MBTD1, Malignant Brain Tumor domain-containing protein 1, is one such PcG protein. MBTD1 is a four MBT repeat protein comprising 628 amino acids. It contains a FCS-type zinc finger at the N-terminus with putative regulatory function and four MBT repeats at the C-terminus. The MBT (Malignant Brain Tumor) repeat is a structural motif of ∼100 amino acids that is conserved from C. elegans to humans and exists as tandem repeats.

To investigate the crystal structure of the four MBT repeat fragment of MBTD1 and characterize its histone binding specificity, we cloned and purified a human MBTD1 fragment composed of all four MBT repeats (residues 130–566). MBTD1130–566 crystallized in the orthorhombic space group P212121 (a = 70.31 Å, b = 100.90 Å, c = 135.30 Å) with two molecules in the asymmetric unit. In the MBTD1 structure, each molecule contains four MBT repeats that exhibit irregular rhomboid architecture. A narrow channel runs through the middle of the structure and is filled with water molecules. Consistent with previously reported MBT repeat structures, each MBT repeat contains an extended “arm” which packs against a globular β subunit core of the preceding repeat. The residues involved in intermolecular hydrogen bond interactions between the two molecules in the asymmetric unit are conserved throughout the whole MBT repeat family, possibly implying that MBTD1 functions as a dimer unit. Although the four MBT repeats of MBTD1 have similar three-dimensional structures and high sequence identity, only the fourth MBT repeat (MBT4) contains the semi-aromatic cage, which is formed by the loops between the first and second strands and the third and fourth strands of the β- barrel core domain and constitutes the binding site for methyllysine residue, analogous to L3MBTL2. The binding pocket of the MBTD1-MBT4 is shown in Figure 4, where an open cage in MBTD1 is formed by aromatic residues Phe526, Trp529, Tyr533, negatively charged Asp502, and Leu508. Interestingly, Arg325 from a symmetry related molecule is inserted into the binding pocket, mimicking the methyl-lysine binding in L3MBTL2. The arginine residue 325 is stabilized by a salt bridge with the pocket residue Asp502, and cation-π and van der Waals and interactions with the aromatic cage residues.

>AKTKAAVSMEGFSWGNYINSNSFIAAPVTCFKHAPMGTCWGDISENVRVEVPNTDCSLPTKVFWIAGIVKLAGYNALLRYEGFENDSGLDFWCNICGSDIHPVGWCAASGKPLVPPRTIQHKYTNWKAFLVKRLTGAKTLPPDFSQKVSESMQYPFKPCMRVEVVDKRHLCRTRVAVVESVIGGRLRLVYEESEDRTDDFWCHMHSPLIHHIGWSRSIGHRFKRSDITKKQDGHFDTPPHLFAKVKEVDQSGEWFKEGMKLEAIDPLNLSTICVATIRKVLADGFLMIGIDGSEAADGSDWFCYHATSPSIFPVGFCEINMIELTPPRGYTKLPFKWFDYLRETGSIAAPVKLFNKDVPNHGFRVGMKLEAVDLMEPRLICVATVTRIIHRLLRIHFDGWEEEYDQWVDCESPDLYPVGWCQLTGYQLQPPASQSSR[2x]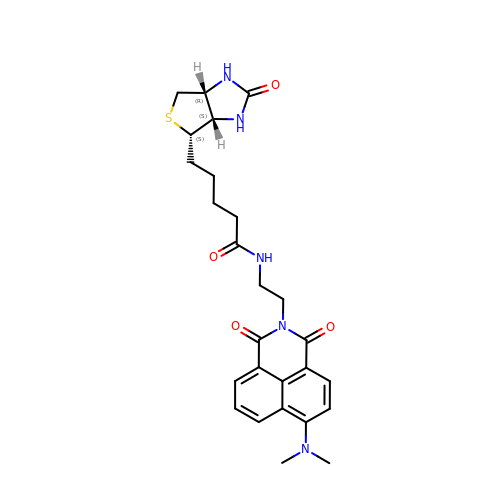5-[(3~{a}~{S},4~{S},6~{a}~{R})-2-oxidanylidene-1,3,3~{a},4,6,6~{a}-hexahydrothieno[3,4-d]imidazol-4-yl]-~{N}-[2-[6-(dimethylamino)-1,3-bis(oxidanylidene)benzo[de]isoquinolin-2-yl]ethyl]pentanamide | C26 H31 N5 O4 S | WAGQBAHKYBJEAZ-LEDOBFOHSA-N>[2x]ELPQMTQQLNSDDMQEQLSATVKFRQILSREHRPPIDVVIQAGVVPRLVEFMRENQPEMLQLEAAWALTNIASGTSAQTKVVVDADAVPLFIQLLYTGSVEVKEQAIWALGNVAGDSTDYRDYVLQCNAMEPILGLFNSNKPSLIRTATWTLSNLCRGKKPQPDWSVVSQALPTLAKLIYSMDTETLVDACWAISYLSDGPQEAIQ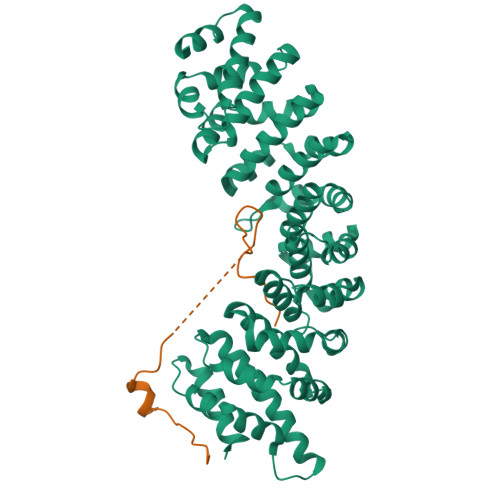AVIDVRIPKRLVELLSHESTLVQTPALRAVGNIVTGNDLQTQVVINAGVLPALRLLLSSPKENIKKEACWTISNITAGNTEQIQAVIDANLIPPLVKLLEVAEDKTKKEACWAISNASSGGLQRPDIIRYLVSQGCIKPLCDLLEIADNRIIEVTLDALENILKMGEADKEARGLNINENADFIEKAGGMEKIFNCQQNENDKIYEKAYKIIETYFGEEEDAVDETMAPQNAGNTFGFGSNVNQQFNF;>[2x]MAKRVADAQIQRETYDSNESDDDVTPSTKVASSAVMNRRKIAMPKRRMAFK>QQVCTTQAETHPALSWSKCTSGGSCTTQAGKVVLDANWRWTHAYPSGNNCYNGNTWDATLCPDDATCAKNCCLEGADYSGTYGVTTSGNQLTIDFVTQSANKNVGARLYLMASDTAYEEFTLLNNEFSFDVDVSALPCGLNGALYFVSMDADGGASKYPTNLAGAKYGTGYCDSQCPRDLKFISGQANVEGWQPSSNNANTGIGGHGSCCSEMDIWEANSISQALTPHPCETVGQVTCSGDDCGGTYSNNRYGGTCDPDGCDWNPYRLGNHTFYGPGSGFTVDTTKKITVVTQFSSTGINRYYVQNGVKFVQPNASGLSGYTGNTINSAYCSAEQTAFGGTSFTDKGGLTQMNKALSGGMVLVLSLWDDYAANMLWLDSTYPTNDTASTPGAARGTCSTSSGVPATVEQQSPNSK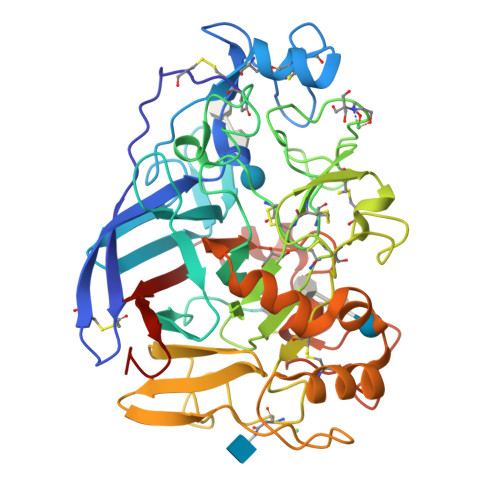VVFSNIKFGPIGSTG[2x]2-(1H-INDOL-3-YL)ACETAMIDE | C10 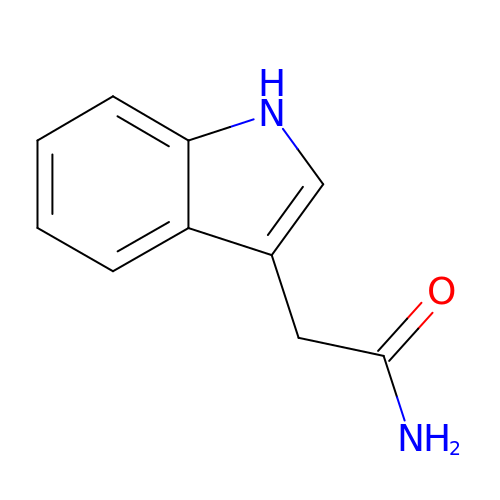H10 N2 O | ZOAMBXDOGPRZLP-UHFFFAOYSA-N>MARDEVRRILPADIKREVLIKDENAETNPDWGFPPEKRPIEMHIQFGVINLDKPPGPTSHEVVAWIKKILNLEKAGHGGTLDPKVSGVLPVALEKATRVVQALLPAGKEYVALMHLHGDVPEDKIIQVMKEFEGEIIQRPPLRSAVKRRLRTRKVYYIEVLEIEGRDVLFRVGVEAGTYIRSLIHHIGLALGVGAHMSELRRTRSGPFKEDETLITLHDLVDYYYFWKEDGIEEYFRKAIQPMEKAVEHLPKVWIKDSAVAAVTHGADLAVPGIAKLHAGIKRGDLVAIMTLKDELVALGKAMMTSQEMLEKTKGIAVDVEKVFMPRDWYPKL[2x];>[2x]MEKQGEKMKRLGKVLHYAKQGFLIVRTNWVPSLNDRVVDKRLQFVGIVKDVFGPVKMPYVAIKPKVSNPEIYVGEVLYVDER;>[2x]MRFRIRKCPKCGRYTLKE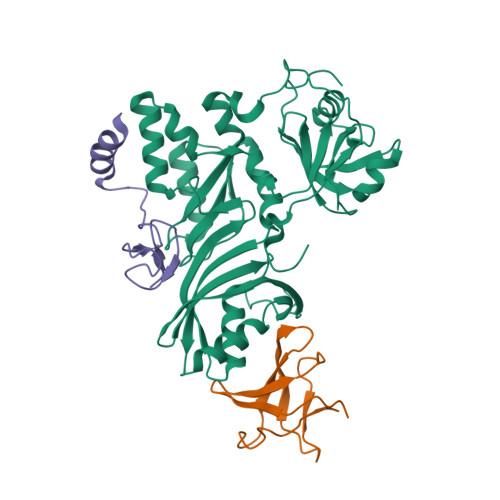VCPVCGEKTKVAHPPRFSPEDPYGEYRRRWKREVLGI The recombinases Rad51 and Dmc1 are highly conserved in the RecA family; Rad51 is mainly responsible for DNA repair in somatic cells during mitosis while Dmc1 only works during meiosis in germ cells. This spatiotemporal difference is probably due to their distinctive mismatch tolerance during HR: Rad51 does not permit HR in the presence of mismatches, whereas Dmc1 can tolerate certain mismatches. Rad51 and Dmc1 sequences are evolutionarily conserved, with Dmc1 about 45% identical to Rad51 in yeast and 54% identical to Rad51 in human. Both are ATPases and require ATP or its non-hydrolysable analogs to assemble on single-stranded DNA (ssDNA) as the presynaptic complex, which leads to searching for homologous double-stranded DNA (dsDNA) in chromosomes. Here, the cryo-EM structures of Rad51–DNA and Dmc1–DNA complexes revealed that the major conformational differences between these two proteins are located in their Loop2 regions, which contain invading single-stranded DNA (ssDNA) binding residues and double-stranded DNA (dsDNA) complementary strand binding residues, stabilizing ssDNA and dsDNA in presynaptic and postsynaptic complexes, respectively.

Using procedures described previously, we obtained cryo-EM structures of the presynaptic and postsynaptic complexes of ScDmc1 wt at the resolutions of 3.2 and 3.4 Å, respectively, and those of hRAD51 wt at 3.0 and 4.0 Å, respectively; these resolutions were higher than for previously reported structures. All four helical assemblies share almost the same right-handed helical symmetry with about 6.3 protomers per turn and a helical pitch of 100 Å. In our models, ssDNA and dsDNA substrates are located in the central axis of the helical structures and stretched to form continuous triplets with DNA bases exposed for homologous pairing and search. In the ScDmc1 presyaptic complex and hRAD51 presynaptic complex with RS-1 which is a compound could enhance the DNA exchange activity, one DNA nucleotide-triplet in a B-form conformation interacts with two consecutive protomers. More specifically, the triplet is sandwiched by Loop2 of ScDmc1-5′ and ScDmc1-0 in the helical axial direction, as well as by Loop1 and Loop2 of ScDmc1-0 in the vertical direction. In ScDmc1, the first phosphate within the triplet is bound by S265 of Dmc1-5′, Q236 and H285 of Dmc1-0, the second phosphate interacts with G283, G284 and R235 of Dmc1-0, and the third phosphate interacts with R223 of Dmc1-0. All of these residues are highly conserved in hRAD51 (22). ScDmc1, which is highly conserved with RecA, ScRad51 and hRAD51, has similar Walker A and B motifs for ATP hydrolysis and the surrounding hydrogen bonds network for coupling of ATP binding and DNA interaction. The EM densities of ScDmc1 reconstructions are sufficient to build atomic models of the intact Loop2, but several residues in the Loop2 of hRAD51 cannot be accounted for in the corresponding reconstructions, indicating a more flexible nature of Loop2 in hRAD51.

>MSVTGTEIDSDTAKNILSVDELQNYGINASDLQKLKSGGIYTVNTVLSTTRRHLCKIKGLSEVKVEKIKEAAGKIIQVGFIPATVQLDIRQRVYSLSTGSKQLDSILGGGIMTMSITEVFGEFRCGKTQMSHTLCVTTQLPREMGGGEGKVAYIDTEGTFRPERIKQIAEGYELDPESCLANVSYARALNSEHQMELVEQLGEELSSGDYRLIVVDSIMANFRVDYCGRGELSERQQKLNQHLFKLNRLAEEFNVAVFLTNQVQSDPGASALFASADGRKPIGGHVLAHASATRILLRKGRGDERVAKLQDSPDMPEKECVYVIGEKGITDSSD[3x]> MHHHHHHENLYFQGMKKEKVEQILAEFQLQEEDLKKVMRRMQKEMDRGLRLETHEEASVKMLPTYVRST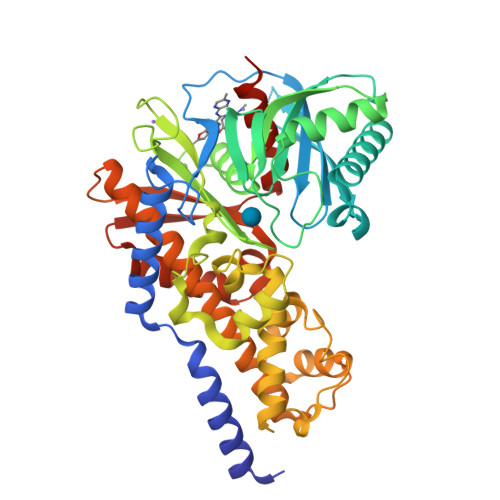PEGSEVGDFLSLDLGGTNFRVMLVKVGEGEEGQWSVKTKHQMYSIPEDAMTGTAEMLFDYISECISDFLDKHQMKHKKLPLGFTFSFPVRHEDIDKGILLNWTKGFKASGAEGNNVVGLLRDAIKRRGDFEMDVVAMVNDTVATMISCYYEDHQCEVGMIVGTGCNACYMEEMQNVELVEGDEGRMCVNTEWGAFGDSGELDEFLLEYDRLVDESSANPGQQLYEKLIGGKYMGELVRLVLLRLVDENLLFHGEASEQLRTRGAFETRFVSQVESDTGDRKQIYNILSTLGLRPSTTDCDIVRRACESVSTRAAHMCSAGLAGVINRMRESRSEDVMRITVGVDGSVYKLHPSFKERFHASVRRLTPSCEITFIESEEGSGRGAALVSAVACKKACMLGQ>REWFLHRNSLIVLADVALFLALYHFLPFEHNVVLGISMLAFIAVLWLTEALHVTVTAILVPVMAVFFGIFETQAALNNFANSIIFLFLGGFALAAAMHHQGLDKVIADKVLAMAQGKMSVAVFMLFGVTALLSMWISNTATAAMMLPLVLGVLSKVDADKQRSTYVFVLLGVAYSASIGGIATLVGSPPNAIAAAEVGLSFTDWMKFGLPTAMMMLPMAIAILYFLLKPTLNGMFELDRAPVNWDKGKVVTLGIFGLTVFLWIFSSPINAALGGFKSFDTLVALGAILMLSFARVVHWKEIQKTADWGVLLLFGGGLCLSNVLKQTGTSVFLANALSDMVSHMGIFVVILVVATFVVFLTEFASNTASAALLIPVFATVAEAFGMSPVL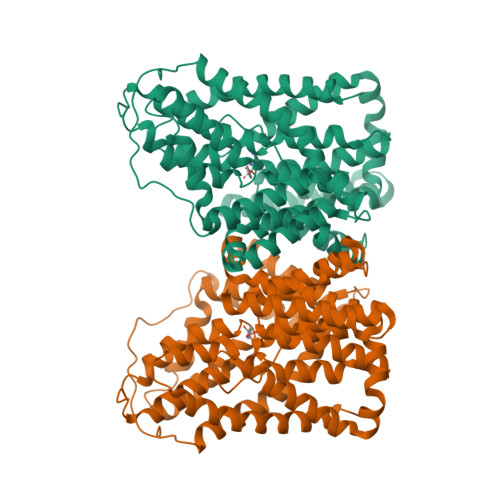LSVLIAVAASCAFMLPVATPPNAIVFASGHIKQSEMMRVGLYLNIACIGLLTAIAMLFWQ[4x]>MAMANNSSVANKVCLIVIDGWGVSEDPYGNAILNAQTPVMDKLCSGNWAQIEAHGLHVGLPEGLMGNSEVGHLNIGAGRVIYQDIVRINLAVKNNKFVTNESLVDACDRAKNGNGRLHLAGLVSDGGVHSHIDHMFALVKAIKELGVPELYLHFYGDGRDTSPNSGVGFLEQTLEFLEKTTGYGKLATVVGRYYAMDRDNRWERINVAYEAMIGGVGETSDEAGVVEVVRKRYAADETDEFLKPIILQGEKGRVQNDDTIIFFDYRADRMREISAAMGMDRYKDCNSKLAHPSNLQVYGMTQYKAEFPFKSLFPPASNKNVLAEWLAEQKVSQFHCAETEKYAHVTFFFNGGLEKQFEGEERCLVPSPKVATYDLQPEMSAAG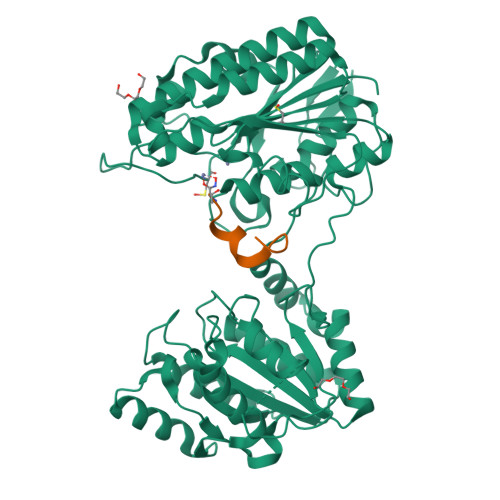VADKMIEQLEAGTHPFIMCNFAPPDMVGHTGVYEAAVKACEATDIAIGRIYEATQKHGYSLMVTADHGNAEKMKAPDGGKHTAHTCYRVPLTLSHPGFKFVDPADRHPALCDVAPTVLAIMGLPQPAEMTGVSIVQKIKLAAALEHHHHHHHHHH[2x];>XYDYPGDHCYLYGTX[2x]>[4x]NRRYDSEFQTMLQHLQPTAENAYEYFTKIATSLFESGINWGRVVALLGFGYRLALHVYQHGLTGFLGQVTRFVVDFMLHHSIARWIAQRGGWVAALNLGNG;>[4x]GGADPKKVLDQAKDQMENVVRTLKQELEELAKEARKLDLTQSEKIELKLRYIVAHLAAIGDIEEAIREAKEEADKLKRAGLVNSQQFDEFKRRLEELHKEADRKRADYAEEFRNKLEYG

BCL-2 protein family members BAK and BAX are the gatekeepers of mitochondrial apoptosis. Homooligomers of BAK and BAX form pores in the mitochondrial outer membrane (MOM) and release apoptotic factors into the cytosol, committing the cell to destruction. We use computational protein design to generate high affinity binders of BAK and BAX with greater than 100-fold specificity for their target. Both binders activate their targets when at low concentration, driving pore formation, but inhibit membrane permeabilization when in excess.

We solved a structure of the BAK:αBAK2 complex in the P1 space group, diffracting to 2.9 Å, with four BAK:αBAK2 heterodimers in the asymmetric unit. The four heterodimeric complexes in the asymmetric unit are similar (between 0.15- and 0.29-Å Cα root mean square deviation (RMSD), 193 to 195 atoms aligned from a total of 197). BAK is in an unlatched conformation with α6 to α8 helices dissociated from the BAK monomer core. The unlatched α6 and α7 helices form a tetrameric BAK crystal contact in the structures, with their hydrophobic faces packing against α4 and α5 helices from a neighboring BAK monomer. No electron density is seen for the BAK α1 and α2 helices. The SDS–polyacrylamide gel electrophoresis (SDS-PAGE) of the crystals shows that the BAK construct is truncated, but only in the crystals and not in solution. The design model of BAK:αBAK2 is very close to the crystal structure, with an all-atom RMSD of 3.2 Å and Cα RMSD of 2.6 Å after alignment of BAK α3 to α5 helices (residues 90 to 141) and αBAK2. The position of BAK helix α3 relative to helices α4 and α5 is shifted by approximately one helical turn in the crystal structure compared to the design model, which was based on NMR structure 2M5B. Despite the α3 shift, the αBAK2 h1-h4 BH3-mimetic residues occupy similar positions at the BAK interface relative to BAK α4 and α5 helices. In conclusion, αBAK2 binds as designed in the BAK BH3-binding groove and can bind to BAK in a partially unfolded, unlatched conformation.> MLRCARVALRADPLNGGSSMTLGSKGSKLSPEPHRRRMPWTAAKEYVPGVVLNARDKMVLDGVQLLDIESIDRASQLDPLEVLRAVVATREYNISTGKNIFQLASQATYNGRGQRFYRKEWQEGTYDKYVTLSAIDFDRDGNKGTAYGYITF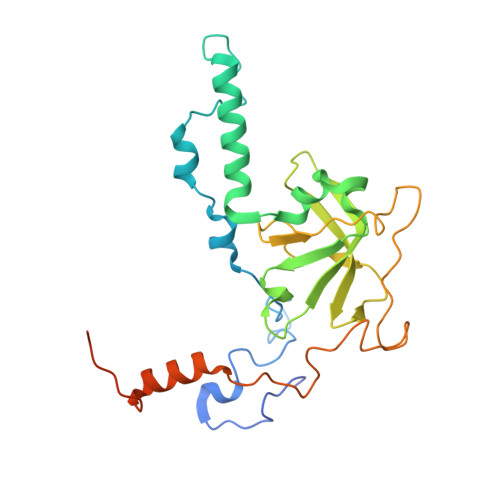HGETTTRPVQVDFADVPGWYMDFVEERAVPFTGIVPPPPSIGTDVPVDPHSYRLKAYPYYDAPNPPEFVERLLKDRGVLPDTPTETADVDKDPTTSDGSVHYDGK>[2x]MTETIPVFDGHNDFLLRLLRNPANRETIWLKGDGTGHLDLPRMKEGGF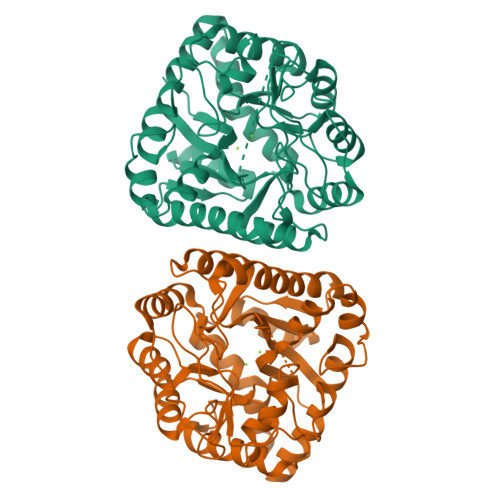AGGFFAIYVPSPQAHDAAHFEAMMDAPPFELPLPPMIRAEQAQPVALAMAGHLLWMERAARGRFKVCRTAAEVRSCHADGIVSGIMHMEGAEAIGADLDALHLFHSLGLRSLGPVWSRPTVFGHGVPFRFPGSPDTGEGLTEAGRRLVAECNRLKIMLDLSHLNEKGFDDVARLSDAPLVATHSNAHAVTPSTRNLTDRQLAMIRESRGMVGLNFATSFLREDGRRSAEMGWEPVLRHLDHLIDRLGEDHVGMGSDFDGATIPQGIADVTGLPALQAAMRAHGYDEPLMRKLCHENWYGLLERSWGA> XE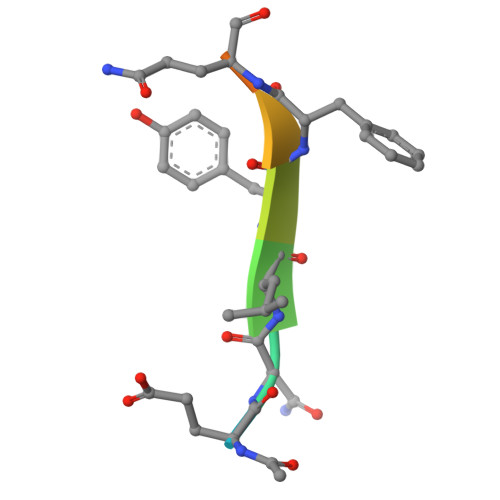NLYFQSGT>[2x]SARLETVQADNIREKKEKLALRQQLNEAKQQLLQQAEYCTEMGAAACTLLWGVSSSEEVVKAILGGDKALKFFSITGQTMESFVKSLDGDVQELDSDESQFVFALAGIVTNVAAIACGREFLVNSSRVLLDTILQLLGDLKPGQCTKLKVLMLMSLYNVSINLKGLKYISESPGFIPLLWWLLSDPDAEVCLHVLRLVQSVVL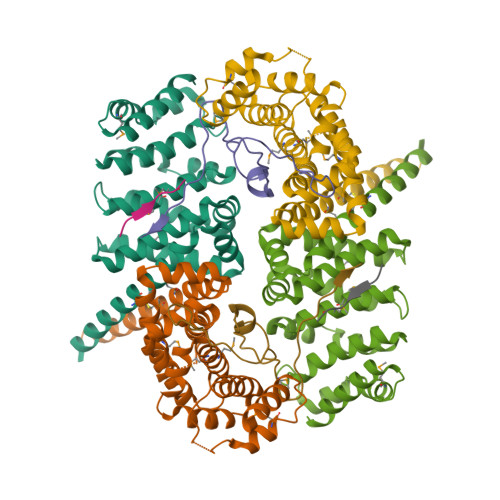EPEVFSKSASEFRSSLPLQRILAMSKSRNPRLQTAAQELLEDLRTLEHNV;>[2x]MKRRGEPLILVGEPSIKRNLLNEFDRIIENQEKSLKASKSTPDGTIKDRRLFMHHVSLEPITCVPF> MALSLCVLFTLASVVSGHVAHPSLGRGDGFPFLWDNAASTLDQLNGTDTTIILNGFNYLDRLSMFKTVLEGTRKYFDSFAPNNTANIYWGFTIYLNWILATGRSADPTGHTTCGLAHGDPMCLAEESWWNCIKYNPAAIAFFAAKKAGIFGDVTKTIVLAKPKEANSPYCSSEEECQAAYPDVMATYLDYFEYLMSLEKTGESIDMDKAQQLLWKAHVTSMENSIAVCKPRLKNYNIIERQLDRDYLISLLYFAATNFPTNFIESIKFVADMPHRQLRFGDIAPFIPDMDMKKN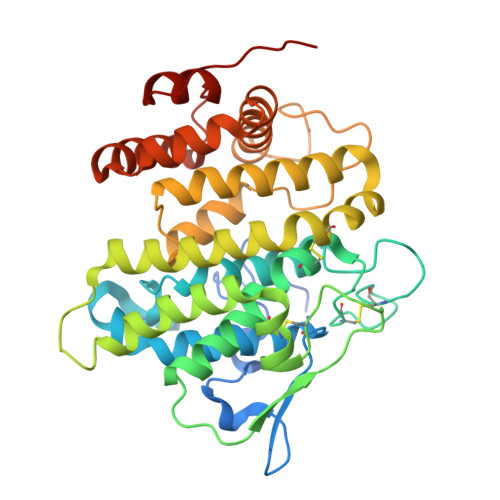NLLVVLHGFYTVHSLSGGSSLTHWRNLMESPVSREMARDMVNLILAGTPVEVQVELAKLGIPTPVDYKDDDK> ADLDQGAQIFEAHCAGCHLNGGN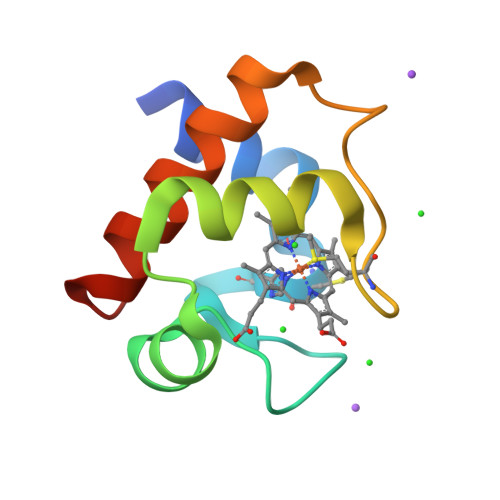IVRRGKNLKKRAMAKNGYTSVEAIANQVTQGKGNMSAYGDKLSSEEIQAVSQYVLQQSQTDWKS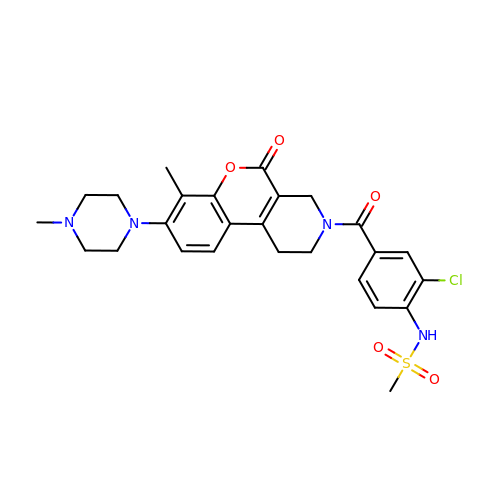N-[2-chloranyl-4-[[7-methyl-8-(4-methylpiperazin-1-yl)-5-oxidanylidene-2,4-dihydro-1H-chromeno[3,4-c]pyridin-3-yl]carbonyl]phenyl]methanesulfonamide | C26 H29 Cl N4 O5 S | DHJUEJALVPLBJH-UHFFFAOYSA-N2-(trimethyl-lambda~5~-arsanyl)ethanol | C5 H14 As O 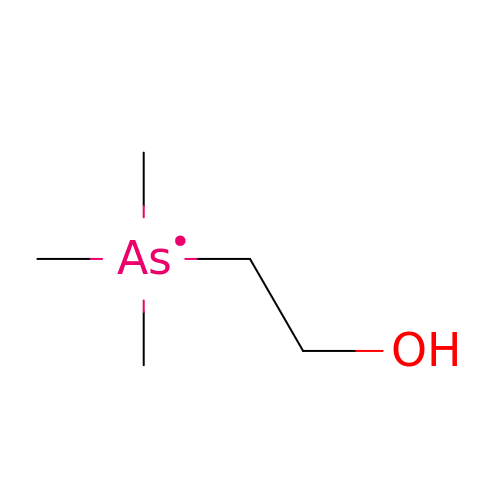| CIHXLIBMYUSRLN-UHFFFAOYSA-N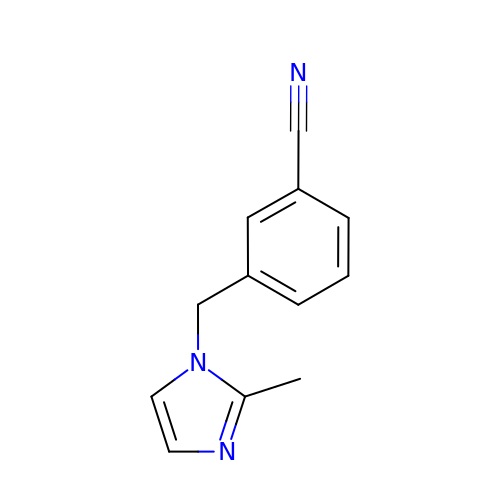3-[(2-methyl-1H-imidazol-1-yl)methyl]benzonitrile | C12 H11 N3 | HMXUYPBDUYSWMA-UHFFFAOYSA-N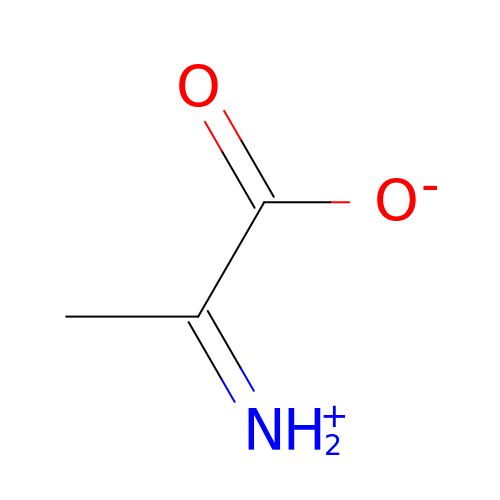AMINO-ACRYLATE | C3 H5 N O2 | DUAWRLXHCUAWMK-UHFFFAOYSA-N[(2~{S},3~{S},4~{R},5~{R})-5-(2-azanyl-7-methyl-6-oxidanylidene-1~{H}-purin-7-ium-9-yl)-3,4-bis(oxidanyl)oxolan-2-yl]methylsulfanyl-[[[(2~{S},3~{S},4~{R},5~{R})-5-(2-azanyl-6-oxidanylidene-3~{H}-purin-9-yl)-3,4-bis(oxidanyl)oxolan-2-yl]methylsulfanyl-oxidanyl-phosphoryl]oxy-sulfanyl-phosphoryl]oxy-phosphinic 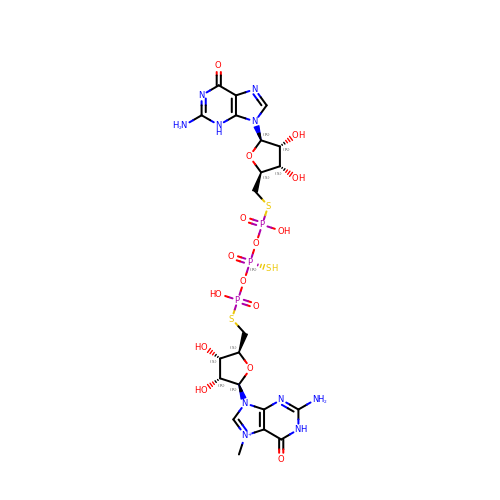acid | C21 H30 N10 O15 P3 S3 | UOUACWJATBZTPY-ACTLBPNMSA-O Coiled-coils are important protein–protein interaction motifs present in ∼3% of all eukaryotic proteins. They consist of two or more amphipathic α-helices that wrap around each other’s hydrophobic seams resulting in parallel or antiparallel filamentous supercoils. Here, we present a case study for the phase determination of coiled-coil structures using a combination of native or engineered cysteine crosslinking together with native SAD phasing. In conclusion, our case study shows that cysteine crosslinking and phasing via sulfur-SAD is a particular useful strategy to solve coiled-coil structures by X-ray crystallography.

The first coiled-coil fragment is derived from CEP135, an important protein implicated in centriole formation. The two-stranded parallel coiled-coil fragment encompasses amino acids 82–144 of human CEP135 (referred to as HsCEP135 82–144) that contains one cysteine and one methionine per monomer. Notably, Cys110 of HsCEP135 82–144 is located in a heptad d core position and has been shown to be able to form a disulfide bridge in the context of its two-stranded parallel coiled-coil structure. Thermal denaturation monitored by CD at 222 nm revealed a broad, non-cooperative unfolding profile typical of monomeric helices. These results suggest that under the conditions tried, HsCEP135 82–144 does not form a coiled-coil structure. The thermal unfolding profile of HsCEP135 82–144 under oxidizing conditions revealed a cooperative unfolding profile (Tm of 62°C) characteristic of a well-folded protein. Taken together, these results demonstrate that HsCEP135 82–144 only forms a two-stranded coiled-coil under oxidizing buffer conditions, while Kif21a_M947C forms a monomeric antiparallel coiled-coil structure under both reducing and oxidizing buffer conditions. The final structure contains two monomers in the asymmetric unit forming a two-stranded, parallel and in-register coiled-coil structure, consistent with the previous structure solved by molecular replacement. A strong peak for the disulfide bridge formed by the cysteine residues at position 110 is visible in the anomalous difference map as well as the signal contributed by the methionines. Though the protein construct ranged from amino acids 82–144 of HsCEP135, only residues 82–134 could be resolved.

>[2x]GSNNELYLELMKLREHSDQHVKELKTSLKKCARETADLKFLNNQYAHKLKLLEKESKAKNERIQQ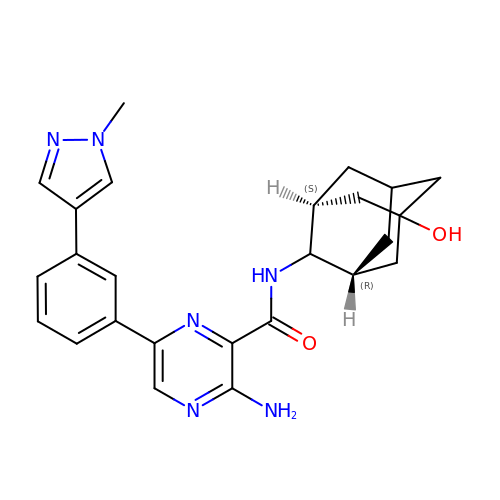3-amino-6-[3-(1-methyl-1H-pyrazol-4-yl)phenyl]-N-[(1R,2r,3S,5s,7s)-5-hydroxyadamantan-2-yl]pyrazine-2-carboxamide | C25 H28 N6 O2 | KADWYJUBGMHRCN-QWOVOEGBSA-N> TF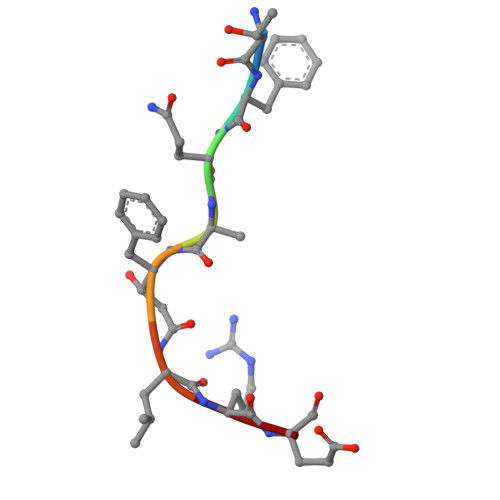QAFLRE>[3x]ADSTEDFPIPRRMIATTCDAEQY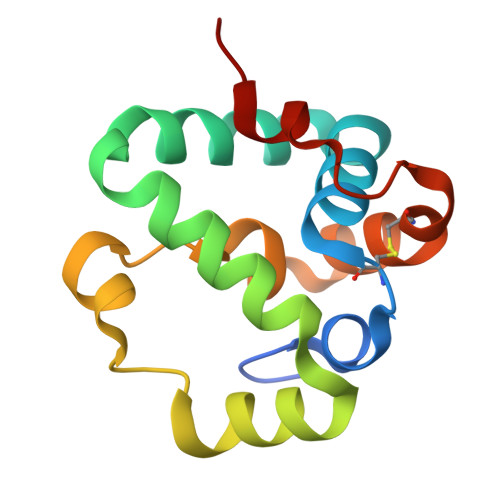LAAVRDTSPVYYQRYMIDFNNHANLQQATINKAHWFFSLSPAERRDYSEHFYNGDPLTFAWVNHMKIFFNNKGVVAKGTEVCNGYPAGDMSVWNWAH> GSVGNREEKILNREIGFAIGMPVCEFDMVKDPEVQDFRRNILNVCKEAVDLRDLNSPHSRAMYVYPPNVESSPELPKHIYNKLDKGQIIVVIWVIVSPNNDKQKYTLKINHDCVPEQVIAEAIRKKTRSMLLSSEQLKLCVLEYQGKYILKVCGCDEYFLEKYPLSQYKYIRSCIMLGRMPNLMLMAKESLYSQLPMDCFTMPSYSRRISTATPYMNGETSTKSLWVINSALRIKILCATYVNVNIRDIDKIYVRTGIYHGGEPLCDNVNTQRVPCSNPRWNEWLNYDIYIPDLPRAARLCLSICSVKGRKGAKEEHCPLAWGNINLFDYTDTLVSGKMALNLWPVPHGLEDLLNPIGVTGSNPNKDTPCLELEFDWFSSVVKFPDMSVIEEHANWSVSREAGFSYSHAGLSNRLARDNELRENDKEQLKAISTRDPLSEITEQEKDFLWSHRHYCVTIPEILPKLLLSVKWNSRDEVAQMYCLVKDWPPIKPEQAMELLDCNYPDPMVRGFAVRCLEKYLTDDKLSQYLIQLVQVLKYEQYLDNLLVRFLLKKALTNQRIGHFFFWHLKSEMHNKTVSQRFGLLLESYCRACGMYLKHLNRQVEAMEKLINLTDILKQEKKDETQKVQMKFLVEQMRRPDFMDALQGFLSPLNPAHQLGNLRLEECRIMSSAKRPLWLNWENPDIMSELLFQNNEIIFKNGDDLRQDMLTLQIIRIMENIWQNQGLDLRMLPYGCLSIGDCVGLIEVVRNSHTIMQIQCKGGLKGALQFNSHTLHQWLKDKNKGEIYDAAIDLFTRSCAGYCVATFILGIGDRHNSNIMVKDDGQLFHIDFGHFLDHKKKKFGYKRERVPFVLTQDFLIVISKGAQECTKTREFERFQEMCYKAYLAIRQHANLFINLFSMMLGSGMPELQSFDDIAYIRKTLALDKTEQEALEYFMKQMNDAHH

Class IA PI3Ks signal downstream of tyrosine kinases, G protein-coupled receptors and small GTPases to regulate cell metabolism, growth, proliferation and migration. They consist of a p110α, β or δ catalytic subunit and a p85 regulatory subunit (further referred to as PI3Kα, PI3Kβ and PI3Kδ), with a broad tissue distribution (p110α, p110β) or enriched in leukocytes (p110δ). PI3Kα phosphorylates PIP2 in the plasma membrane to PtdIns(3,4,5)P3 (or PIP3), which can be converted by 5-phosphatases to PtdIns(3,4)P2. Here we report on the discovery of UCL-TRO-1938 (further referred to as 1938), a small molecule activator of the PI3Kα isoform, a critical effector of growth factor signalling.

We next used a deletion variant of p110α (p110α AA105-1048)30 in which the p85 adaptor-binding domain (AA1-104) and a C-terminal membrane binding motif in the kinase domain (AA1049-1068) were deleted. Co-crystallisation with 1938 did not yield crystals, however, soaking preformed crystals with 1938 revealed density for 1938. The bound 1938 is in a pocket surrounded by residues E365, I459, L540, D603, C604, N605, Y641 of p110α and, in agreement with HDX-MS protection, S1003, L1006, G1007 and F1016. The acetylated indoline of 1938 sits in a pocket comprised of L1006, F1016 and I459, and makes face-to-edge interactions with F1016. Two orientations for the indoline group of 1938 fit the density equally well (yellow and magenta sticks in Extended Data Fig. 2f), and both orientations have an internal H-bond between the oxygen of the acetylated indoline and the NH group connecting the indoline to the pyridine. However, in one orientation (magenta carbons) the compound is less strained, with a better internal H-bond geometry, so this is our preferred model.Binding of 1938 induces F1016 to move away from the pocket in order to accommodate the ligand. The piperazine is surrounded by E365 and L540, and points out towards solvent. 1938 induced global conformational shifts in the p110α crystal structure, with the C2 and helical domains moving away from the kinase domain, the AA1002-1016 kinase/activator interface moving away from the helical domain and the α-helix AA1016-1026 moving toward the active site. Activation loop residues K942 and R949 are important for recognizing PIP232, suggesting that a component of the mechanism of action of 1938 is to cause repositioning of the activation loop to facilitate productive phosphotransfer to PIP2. In addition, 1938 binding causes pivoting of the helical domain to bring the ATP-binding loop and the N-lobe of the kinase domain towards the ATP-binding pocket.>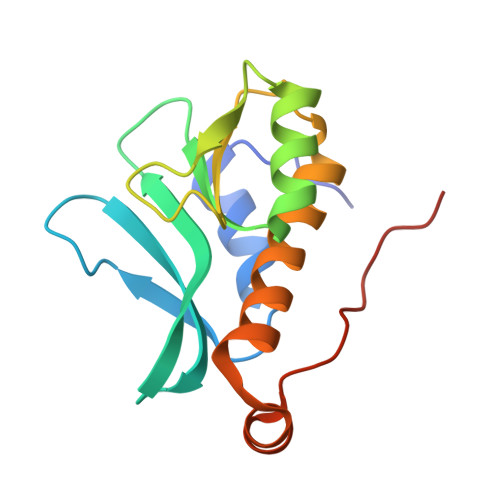 MSLQTPMQTVDDLRSVCDELPHSLETFPFDDETLVFKVGYLSKSRMYALTDITQDPLRLSLKVDPERGEELRQAHPQSIAPGYHLNKKHWVTVTLDGTVPAELLGELLRGSYLLVTKKGFTKAERKELGLPDSLEGGSHHHHHH>MDAKKVAKKAAIQAARRITELAQVLVELLKEALKLDLTQEMRKKLIERYAAAIIRAIGDINNAIYQAKQEAEKLKKAGLVDSDQLDALLRALDELQKVASKAANQLGRLFEEALKRLDKDNGGEEEKDRTAKWFEFEARAIEIALRLAAIGDVFDLEKEWRKLK[2x];>[4x]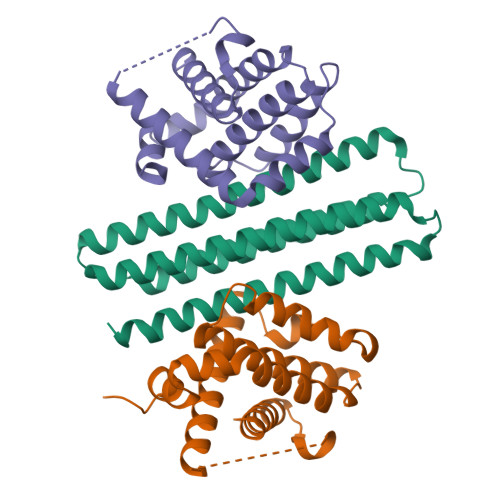GHMMSQSNRELVVDFLSYKLSQKGYSWSQFSDVEENRTEAPEGTESEAVKQALREAGDEFELRYRRAFSDLTSQLHITPGTAYQSFEQVVNELFRDGVNWGRIVAFFSFGGALCVESVDKEMQVLVSRIAAWMATYLNDHLEPWIQENGGWDTFVELYGNNAAAESRKGQER> ISAAAFDAAEQLIQVWDGTPEALVFEATEDEVAEYLSAVDVAIEHLARGSGGGAGGAGSSSSSTAGRAGVAVQLAMARLEEELRHLMVRHAVPLDPTGLFFSLRRLSLGSMDDLDTSSEFDAATPHSIDVAPETARGGPLVNPFEDQVFDPVRPEAVDDLRAIADRMARAGYSRELADAYCGIRRDLLDEYLSALGVERLSIDEVQRIEWKHLNDKMKKWVQAVKTVVRVLLAGERRLCDQVLSVSDELREECFIESTKGCIMQILSFGDAVAVCPRSPEKLSRILDMYEALAEVIPEMKDLCLGSSGDGVISDVQANLDRLGDAIRGTLFEFGKVLQLESSRRAMTAGEIHPMTRYVMNYLRLLVVYSDTLDALLDDNADDQIDLARAEDQDQEHLESMTPLGKRLLKLISYLEANLEEKSKLYEDSALECIFSMNNLLYIVQKVRDSELGKILGDHWVKRRNGKIRQYSKSYLRISWMKVLSFLKDDGHGSGSGSSSGSGSGHSSSRMSIKEKFKNFNLAFEEIYRNQTTWKVPDPQLREELKISISENVIPAYRAFLGRYGSQVDGGRNSGKYIKYTPEDLESQLSD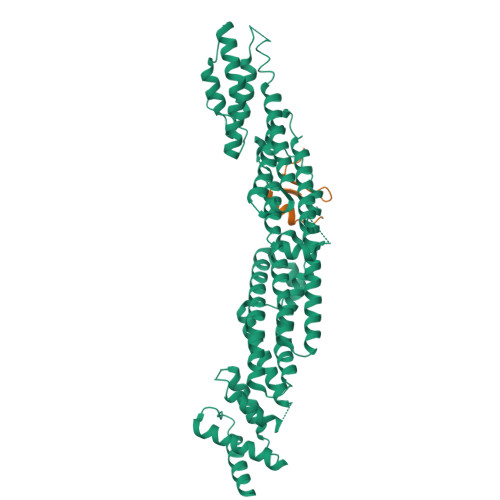LFEGAPGPANHSRRRT;> LPTPASLNGNTEVATISDVKLEARSDTTYHKCSKCGYGSDDSDAYFNHKCN> SPSVEACGYSDRVAQLTVGNSSITTQEAANIVLAYGEWPEYCPDTDATAVDKPTRPDVSVNRFYTLDSKMWQENSTGWYWKFPDVLNKTGVFGQNAQFHYLYRSGFCLHVQCNASKFHQGALLVAVIPEFVIAGRGSNTKPNEAPHPGFTTTFPGTTGATFHDPYVLDSGVPLSQALIYPHQWINLRTNNCATVIVPYINAVPFDSAINHSNFGLIVIPVSPLKYSSGATTAIPITITIAPLNSEFGGLRQAV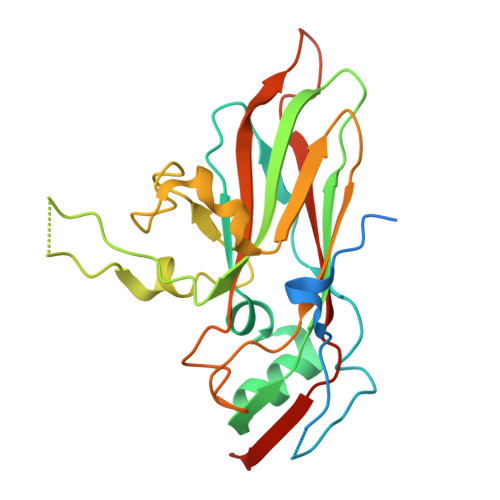SQ Glutathione transferases (GSTs; EC 2.5.1.18) represent a ubiquitous multigenic family of enzymes that conjugate the reduced tripeptide glutathione (GSH, γ-Glu-Cys-Gly) on a wide range of endogenous and exogenous electrophilic molecules. At the structural level, GSTFs exist as homodimers, the dimerization interface involving mainly hydrophobic surface patches. Each monomer comprises an active site region formed by a glutathione binding pocket (G-site) primarily involving residues from the conserved N-terminal thioredoxin domain and an hydrophobic pocket (H-site) primarily involving residues from the less conserved C-terminal domain. A PttGSTF1 monomer consists of an N-terminal domain (β1α1β2α2β3β4α3) and a C-terminal domain composed of α-helices (α4α5α6α6′α7α8) as classically observed in most GST classes.

The analysis of the Fourier difference maps of PttGSTF1 revealed the presence of two ligands in the active site in each monomer: a glutathione molecule originating from the pre-treatment performed with an excess of GSH and a MES molecule present in the crystallization buffer. They are located respectively in the G and H sites. Currently, we do not have any evidence for a GSH-conjugation reaction with MES nor data for any non-catalytic binding. Both glutathione and MES molecules were refined with complementary occupancies. Therefore, PttGSTF1 structure can be described as two structures: PttGSTF1 in complex with glutathione and PttGSTF1 in complex with a MES molecule. In PttGSTF1, a glutathione molecule is positioned in the G site groove which is mainly populated by polar residues from the N-terminal domain. The thiol group of the cysteine of the GSH moiety is quasi-equidistant to the hydroxyl groups of Ser13 and Thr14 (3.2 and 3.4 Å respectively). While Ser13 likely corresponds to the catalytic residue found in most GSTFs and is the primary candidate for GSH activation, the hydroxyl group of the adjacent Thr14 is found approximately at the same distance in the PttGSTF1 structure. With regard to the electrophilic substrate site, a MES molecule occupies the position adopted by other substrates in known GSTF structures. The MES molecule is surrounded by the hydrophobic residues Leu12, Leu37 and Phe123. Moreover, the oxygen atom of the morpholino ring is hydrogen-bonded to the NH and OH groups of Thr14 and the sulfonic group forms a salt bridge with His119.

>MATPVTIYGPPLSTAVSRVLATLIEKDVPFHLIPIDLSKGEQKKPEYLKIQPFGQVPAFKDESITLFESRAICRYICDKYADKGNKSLYGTDILSKANIDQWVETDGQTFGPPSGDLVHDLLFSSVPVDEALIKKNVDKLAKVLDIYEQKLGQTRFLAGDEFSFADLSHLPNGDYLVNSTDKGYLFTSRKNVNRWWTEISNRESWKKVLEMRKNA[2x]> ELLEGELKTAALAQHDEAMGGSLRRKGESVKKRLVSGTAASLQELSLQPSSNGIASAGKSEDGEAGDGMSGEFGAALTDSNVENNVKAFDLIFTKLKSTNQLERVAASYELKSCLISLAREVSTEYFQRFSNDINNKVFELIHGTDSNEKLGGVLAVDTLIDFYSHTDELPNQTSRLANYLRVLIPSNDIEVMRAAATTLGKLAVPGGTLTSEFVEFEVKTCIEWLTTSPESSSSNSKQEYRKHASLLIISSIAHNSPYLLYPFVNSILDNIWRALRDTKLVIRTDAAVTLGKCLTIINDRDSSLTKKWVQRLFNGCIYGLQLNTTVSIHGTLLVYRQLVSLEGGYLKDKYEEIYETTMKHRDNKNIIIRKEIYAIIPVLAAFDPKLFTQKYLDATMIHYLTLLKNMTSHQIALSDKGPILVSIGDIAYHVGSEIGPYLDAIVENLRDGLETKFKTRKEFEKDIFYCVSKLACAVRPLLAKYLNRGLLDALLACPLSDHMQETLLVICEKIPSMEVTVNEKLLNIICLVLS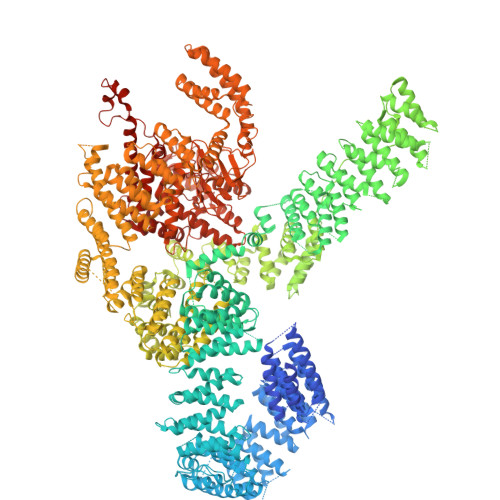GEKFRPPGSPTPMKSLSSETARAYRDQSLLRKTGENNNDTLDAMILRKALRMLSDIKPKYSLTEFIRRVIISYMEHDNMQVRKLAALTSCDLFVKDSICKQTSLYALNVVSEVLSKLLTVAITDPVAEIRLEILKHLDRNFDPQLSQPDNTKLLFMALNDEVFAIQMEAMKICGRLALVNPAYVIPSLRKTLIQLLTELKHSKMTRKKEECASLLCTLISSSSDVTKPYLEPVIEILLPKSQDPSSAVASTALKALGEISVVGGEDMLPFLDELMPLIIDTFQDQSNSFKRGAALKALGQLAASSGYVIDPLLDYPELLGVLINILKSESSQNIRRETVRLIGILGALDPYKHREVERTSITNITSEQNAPPIDVALLMQGMSPSNEEYYPTVVIGVLMKILKDPSLSIHHSTVIQAIMHIFQTMGLRCVIFLKQIIPGFILVMHTCPPSLLELYFQQLSVLISIVKQHIRPHVTEIVDVISEFFPVLKLQLTIISVIESLSRALEGEFNPHLPTILSLFLDVLEKDQSNKKVVSVRILKSLVVFGPHLEEYVHLVLPTIIKLSEFSSGNLKKAAIITIGRLSKNVNALEMSSRIVQALVRVLNTSETEYVKATMNTLSLLLLQLNIDFTVFIPVINKTLVKQNIQHTIYDRLVAKLLNNEPLPTKIIIDKDFDLPNKEMDDVKVASKKLPVNQMVLKNAWDCSQQRTKEDWQEWIRRLSISLLKESSSHALRACSGLAGIYYPLARELFNASFASCWGELYTQYQEDLIQSLCAALSSPNNPPEIHQTLLNLVEFMEHDDKPLPISISTLGEYAQRCHAYAKALHYKELEFIEEPSTSTIESLITINNQLHQTDAAIGILKHAQQHHDLQLKETWYEKLQRWDDALNAYNKREAAGEDSVEVTIGKMRSLHALGEWDQLSELAADKWASSQLEVKRAIAPLAAGAAWGLAQWDRVEQYIEVMKPQSPDKAFFDAILCLHRNNFEKAAEHIFSARDLLVTEMSALVNESYNRAYGVVVRTQMVAELEEIIQYKKLPQGSERRAMIRKTWNKRLLGCQKNVDVWQRVLKVRSLVIKPKQDMKVWIKFANLCRKSGRLGLAQKTLNTLLEESGDPKNPNTARAPPPVVYAQLKYMWATGSQKEALNHLISFTSRMAHDLGLDPSNMIAQSVPQNSSVSQHHIEDYTKLLARCFLKQGEWRVSLQPNWRLENPDAILGSYLLATHFDKTWYKAWHNWALANFEVTSSLTQRIKDDKVPPTLEDASTEFTNGAVAGLNANDNFPPELVQRHVVPAIKGFFHSIALSQSSSLQDTLRLLTLWFKFGGIPEAAQAMHEGFGLIKIDNWLEVIPQLISRIHQPNQTVSRSLLSLLADLGKAHPQALVYPLTVAIKSDSVSRQRAALSIIDKMRMHSPKLVNQAELVSDELIRVAVLWHELWYEGLEDASRQFFGEHNTEKMFATLEPLHEMLKRGPETLREISFQNSFGRDLNDAYEWVLNYKRTKDINNLNQAWDIYYNVFRRISRKLPQLQTLDLQHVSPKLSAAKDLELAVPGTYHAGKPIVRITHFEPVFTVISSKQRPRRVIIKGSDGKDYQYLLKSHEDIRQDNLVMQLFGLVNTLLQNDPESFQRHLNIQQYPAIPLSPKTGLLGWVPNSDTFHVLIREHREASKIPLNIEHRIMLQMAPDYDNLTLLQKVEVFTYALDNTKGQDLYKVLWLKSRSSESWLDRRTTYTRSLAVMSMVGYILGLGDRHPSNLMLDRITGKVVHIDFGDCFEAAILREKYPEKVPFRLTRMLTYAMEVSGIEGSFRITCENVMMVLRDNKESLMAILEAFAYDPLINWGFDLPTHAVMEQTGIDLPLANPSELLRKGVISVEDAAKMELQQKAEVRNARATLVLKRIADKLTGNDFPRCQELSVPDQVDKLIQQATSVENLCQHYIGWCSFW3-(4-phenoxyphenyl)-1-[(3S)-piperidin-3-yl]-1H-pyrazolo[3,4-d]pyrimidin-4-amine | C22 H22 N6 O | 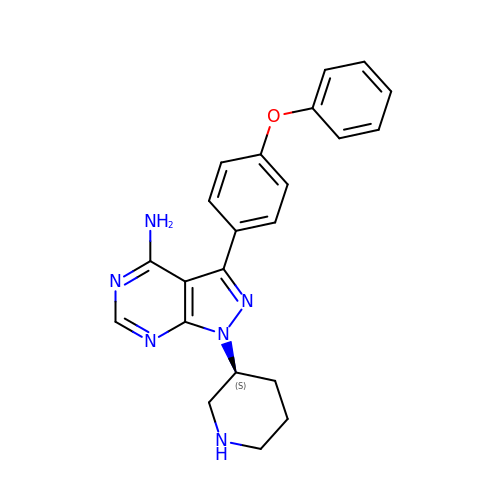GPSQYTDPBDNDGI-INIZCTEOSA-N> DQAGKSPNAVRY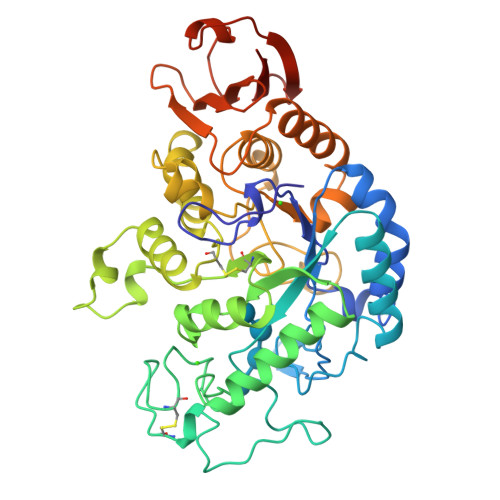HGGDEIILQGFHWNVVREAPNDWYNILRQQAATIAADGFSAIWMPVPWRDFSSWSDGSKSGGGEGYFWHDFNKNGRYGSDAQLRQAASALGGAGVKVLYDVVPNHMNRGYPDKEINLPAGQGFWRNDCADPGNYPNDCDDGDRFIGGDADLNTGHPQVYGMFRDEFTNLRSQYGAGGFRFNFVRGYAPERVNSWMTDSADNSFCVGELWKGPSEYPNWDWRNTASWQQIIKDWSDRAKCPVFDFALKERMQNGSIADWKHGLNGNPDPRWREVAVTFVDNHDTGYSPGQNGGQHHWALQDGLIRQAYAYILTSPGTPVVYWDHMYDWGYGDFIRQLIQVRRAAGVRADSAISFHSGYSGLVATVSGSQQTLVVALNSDLGNPGQVASGSFSEAVNASNGQVRVWRSGTGSGGGEPGA>[2x]MSEQLVTPENVTTKDGKINLLDLNRQQMREFFKDLGEKPFRADQVMKWMYHY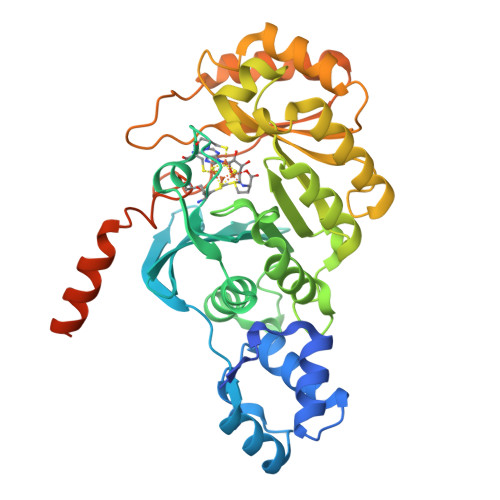CCDNFDEMTDINKVLRGKLKEVAEIRAPEVVEEQRSSDGTIKWAIAVGDQRVETVYIPEDDRATLCVSSQVGCALECKFCSTAQQGFNRNLRVSEIIGQVWRAAKIVGAAKVTGQRPITNVVMMGMGEPLLNLNNVVPAMEIMLDDFGFGLSKRRVTLSTSGVVPALDKLGDMIDVALAISLHAPNDEIRDEIVPINKKYNIETFLAAVRRYLEKSNANQGRVTIEYVMLDHVNDGTEHAHQLAELLKDTPCKINLIPWNPFPGAPYGRSSNSRIDRFSKVLMSYGFTTIVRKTRGDDIDAACGQLAGDVIDRTKRTLRKRMQGEAIDIKAVGNSSSVDKLAAALEHHHHHH> MAHHHHHHMSDNPHSLHPLSSDSTSQALHSSTKPPATPHEGEFHSVRDSNVVEPTEANGKKSHVGPHLGSRMRIYEYSIEHNDAFWAEIARRDFYWKTTWPDDQHVKSYNFDKSKGPIFVKWFEGAVTNVCYNALDRHLPAHKDRVCFYFEGNDPSVTEAVTYGSMYTRVVELANVLKYQYGIAKGDRVGLYLPMIPFAAVAMLACARIGAVITVIFGGFSAQALSSRLKDAQTKLLITADASARGTKPIPLKDVADEALKECEEEGMSIACLVAENMNRQSCKMKEGRDTWYGDALARLTPEQHEECPVEWMDAEDVLFLLYTSGSTGKPKAIVHTTAGYMVYASTTFMYSFDYHMDDVYFCTADIGWITGHSYVVYGPMIHCATSVLFEGVPNYPDYSRWWQLVEKYKVSILYTAPTAIRSLMQAGDDYVKVGNRSTLRVLGSVGEPINVEAWKWLRDVGGEGHCDVSDTWWQTETGGHMITPMPGCTPMKPGSATLPFFGVQPVILDPMKLHEKQGPAEGLLAIRAPWPGMARTIYGDHARFEKTYFGVDGYYMTGDGARRDSDGYYWITGRVDDVLNVSGHRIGTSEIEDAVNTHPAVVESA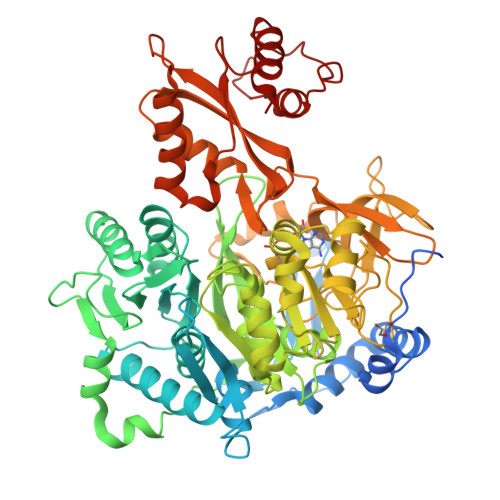VVGFPHNIKGEGIYVFLTFRQGTEVTPELLAAVKATVRKVIGPLATPDVMQVARVGLPKTRSGKIVRRILRKVSAGQYTELGDTSTLANPDVVEDLIAEHQRLCSQN>[2x]MSLADAVAHLTPERWEEANRLLVRKALAEFTHERLLTPEREPDDGGGQTYVVRSDDGQTAYRFTATVRALDHWQVDAASVTRHRDGAELPLAALDFFIELKQTLGLSDEILPVYLEEISSTLSGTCYKLTKPQLSSAELARSGDFQAVETGMTEGHPCFVANNGRLGFGIHEYLSYAPETASPVRLVWLAAHRSRAAFTAGVGIEYESFVRDELGAATVDRFHGVLRGRGLDPADYLLIPVHPWQWWNKLTVTFAAEVARGHLVCLGEGDDEYLAQQSIRTFFNASHPGKHYVKTALSVLNMGFMQGLSAAYMEATPAINDWLARLIEGDPVLKETGLSIIRERAAVGYRHLEYEQATDRYSPYRKMLAALWRESPVPSIREGETLATMASLVHQDHEGASFAGALIERSGLTPTEWLRHYLRAYYVPLLHSFYAYDLVYMPHGENVILVLADGVVRRAVYKDIAEE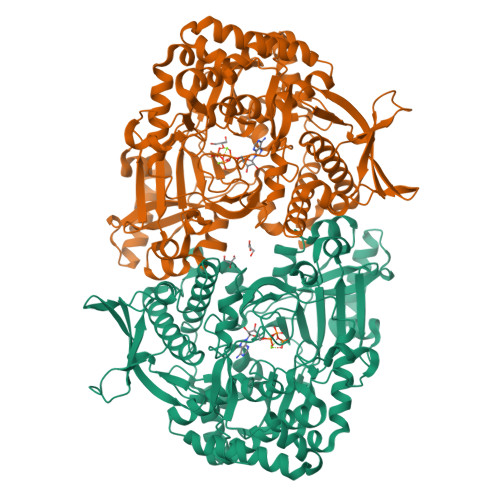IAVMDPDAVLPPEVSRIAVDVPDDKKLLSIFTDVFDCFFRFLAANLAEEGIVTEDAFWRTVAEVTREYQESVPELADKFERYDMFAPEFALSCLNRLQLRDNRQMVDLADPSGALQLVGTLKNPLAGRLQHHHHHH> GYKERVERLCKSKELFEERLGLEIRRIHNEQLQFIFRHIDHKDPDK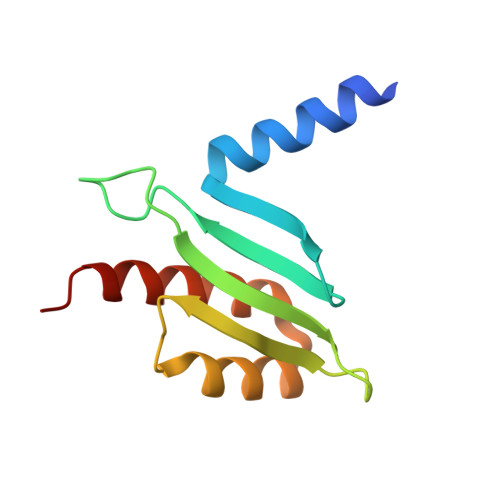PYMFTLSINEQGDYEVTSCTPPLDCISEFQLKVRETNNFSAFIANIRKAFTALSFKQST>PYVEIIEQPKQRGMRFRYKCEGRSAGSIPGERSTDTTKTHPTIKINGYTGPGTVRISLV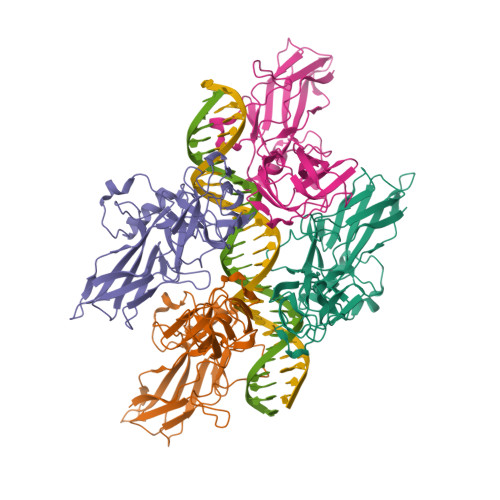TKDPPHRPHPHELVGKDCRDGYYEADLCPDRSIHSFQNLGIQCVKKRDLEQAISQRIQTNNNPFHVPIEEQRGDYDLNAVRLCFQVTVRDPAGRPLLLTPVLSHPIFDNRAPNTAELKICRVNRNSGSCLGGDEIFLLCDKVQKEDIEVYFTGPGWEARGSFSQADVHRQVAIVFRTPPYADPSLQAPVRVSMQLRRPSDRELSEPMEFQYLPD[4x]> MVAKKWVYYFGGGNADGNKNMKELLGGKGANLAEMVNLGIPVPPGFTITTEACKTYQETETIPQEVADQVRENVSRVEKEMGAKFGDPANPLLFSVRSGAAASMPGMMDTVLNLGLNKVTVDAWVRRAPRLERFVYDSYRRFITMYADIVMQVGREDFEEALSRMKERRGTKFDTDLTASDLKELCDGYLELFELKTGCSFPQDPVMQLFAAIKAVFRSWGNPRATIYRRMNNITGLLGTAVNVQAMVF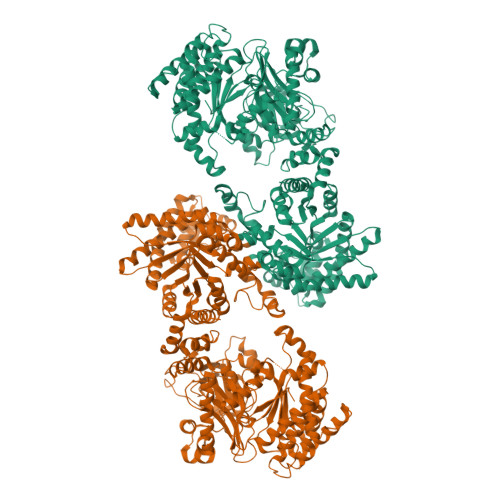GNINDRSATGVAFSRSPSTGENFFFGEYLVNAQGEDVVAGIRTPQQINHSLSLRWAKAHGVGEEERRKRYPSMEEAMPENYRLLCDVRKRLENHYRDMQDLEFTVQDGRLWLLQCRNGKRTIHAAVRIAIDMVNEGLISREEAVLRIDPYQVDHLMHPNLEPGAEKANKPIGRGLAASPGAAVGQVVFDAESAKEWSGRGKKVIMVRLETSPEDLAGMDAACGILTARGGMTSHAAVVARGMGKCCVSGCGDMVIRGKSFKLNGSVFREGDYITIDGSKGLIYAGKLKLRSPDLKGSFQTILQWCQEMKRLGVRTNADTPADAAKARSFGAEGVGLCRTEHMFFEGSRINFIREMILADSASGRKAALDKLLPIQRADFVGILRAMRGLPVTIRLLDPPLHEFVPHDAAAQFELAQKLGMPAEKVRNRVNALHELNPMLGHRGCRLGITYPEIYNMQVRAIIEAAIAVSEEGSSVIPEIMVPLVGKKEELSLIREEVVKTAEAVITKSGKRVHYTVGTMIEVPRAAVTADSIAQKADFFSFGTNDLTQMGCGFSRDDAGPFLRHYGNLGIYAQDPFQSIDQEGIGELVRIAVTKGRRVKPMLKMGICGEHGGDPATIGFCHKVGLDYVSCSPFRVPVAIVAAAHASIKDRRAAMKARKGFAAKL>AEKLPKAPVITTPLETVDALVEEVATFMCAVESYPQPEISWTRNKILIKLFDTRYSIRENGQLLTILSVEDSDDGIYCCTANNGVGGAVESCGALQVKMKPKITRPPINVKIIEGLKAVLPCTT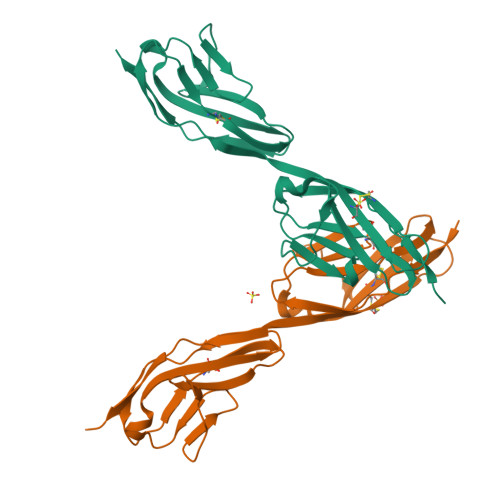MGNPKPSVSWIKGDSALRENSRIAVLESGSLRIHNVQKEDAGQYRCVAKNSLGTAYSKLVKLEVEVFA[2x]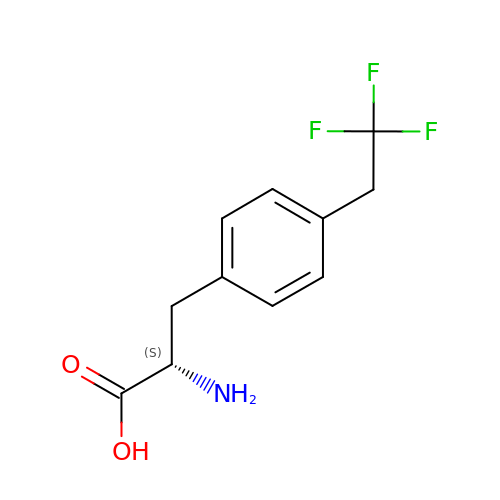4-(2,2,2-TRIFLUOROETHYL)-L-PHENYLALANINE | C11 H12 F3 N O2 | VXIZYDKGLBPCAQ-VIFPVBQESA-N(2R)-2-[4-(4-cyano-2-fluorophenoxy)phenoxy]propanoic 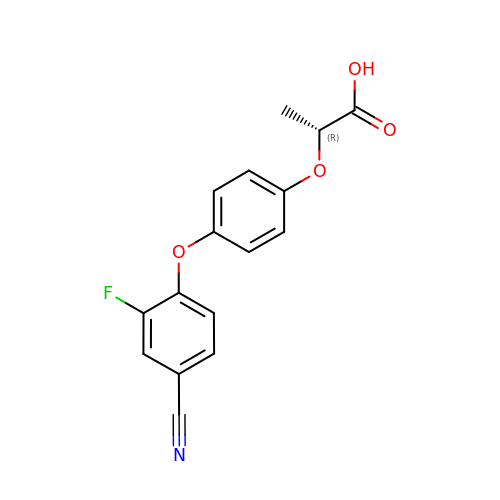acid | C16 H12 F N O4 | ROBSGBGTWRRYSK-SNVBAGLBSA-N> MDALCGSGELGSKFWDSNLSVHTENPDLTPCFQNSLLAWVPCIYLWVALPCYLLYLRHHCRGYIILSHLSKLKMVLGVLLWCVSWADLFYSFHGLVHGRAPAPVFFVTPLVVGVTMLLATLLIQYERLQGVQSSGVLIIFWFLCVVCAIVPFRSKILLAKAEGEISDPFRFTTFYIHFALVLSALILACFREKPPFFSAKNVDPNPYPETSAGFLSRLFFWWFTKMAIYGYRHPLEEKDLWSLKEEDRSQMVVQQLLEAWRKQEKQTARHKASAAPGKNASGEDEVLLGARPRPRKPSFLKALLATFGSSFLISACFKLIQDLLSFINPQLLSILIRFISNPMAPSWWGFLVAGLMFLCSMMQSLILQHYYHYIFVTGVKFRTGIMGVIYRKALVITNSVKRASTVGEIVNLMSVDAQRFMDLAPFLNLLWSAPLQIILAIYFLWQNLGPSVLAGVAFMVLLIPLNGAVAVKMRAFQVKQMKLKDSRIKLMSEILNGIKVLKLYAWEPSFLKQVEGIRQGELQLLRTAAYLHTTTTFTWMCSPFLVTLITLWVYVYVDPNNVLDAEKAFVSVSLFNILRLPLNMLPQLISNLTQASVSLKRIQQFLSQEELDPQSVERKTISPGYAITIHSGTFTWAQDLPPTLHSLDIQVPKGALVAVVGPVGCGKSSLVSALLGEMEKLEGKVHMKGSVAYVPQQAWIQNCTLQENVLFGKALNPKRYQQTLEACALLADLEMLPGGDQTEIGEKGINLSGGQRQRVSLARAVYSDADIFLLDDPLSAVDSHVAKHIFDHVIGPEGVLAGKTRVLVTHGISFLPQTDFIIVLADGQVSEMGPYPALLQRNGSFANFLCNYAPDEDQGHLEDSWTALEGAEDKEALLIEDTLSNHTDLTDNDPVTYVVQKQFMRQLSALSSDGEGQGRPVPRRHLGPSEKVQVTEAKADGALTQEEKAAIGTVELSVFWDYAKAVGLCTTLAICLLYVGQSAAAIGANVWLSAWTNDAMADSRQNNTSLRLGVYAALGILQGFLVMLAAMAMAAGGIQAARVLHQALLHNKIRSPQSFFDTTPSGRILNCFSKDIYVVDEVLAPVILMLLNSFFNAISTLVVIMASTPLFTVVILPLAVLYTLVQRFYAATSRQLKRLESVSRSPIYSHFSETVTGASVIRAYNRSRDFEIISDTKVDANQRSCYPYIISNRWLSIGVEFVGNCVVLFAALFAVIGRSSLNPGLVGLSVSYSLQVTFALNWMIRMMSDLESNIVAVERVKEYSKTETEAPWVV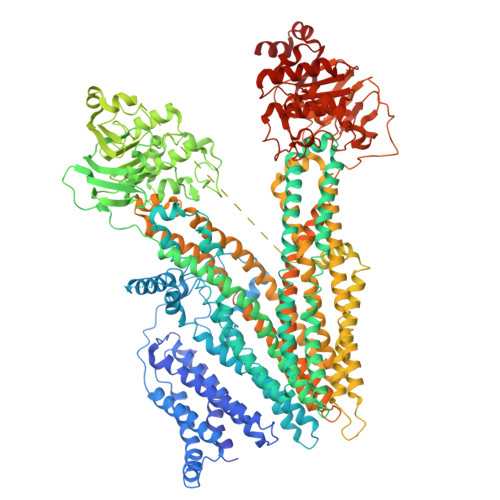EGSRPPEGWPPRGEVEFRNYSVRYRPGLDLVLRDLSLHVHGGEKVGIVGRTGAGKSSMTLCLFRILEAAKGEIRIDGLNVADIGLHDLRSQLTIIPQDPILFSGTLRMNLDPFGSYSEEDIWWALELSHLHTFVSSQPAGLDFQCSEGGENLSVGQRQLVCLARALLRKSRILVLDEATAAIDLETDNLIQATIRTQFDTCTVLTIAHRLNTIMDYTRVLVLDKGVVAEFDSPANLIAARGIFYGMARDAGLA>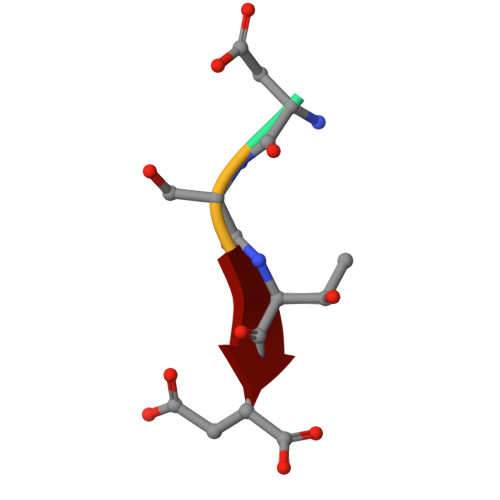 DSTD> GSHTAEEDMEDDTSWRSEATFQFTVERFSRLSESVLSPPCFVRNLPWKIMVMPRFYPDRPHQKSVGFFLQCNAESDSTSWSCHAQAVLKIINYRDDEKSFSRRISHLFFHKENDWGFSNFMAWS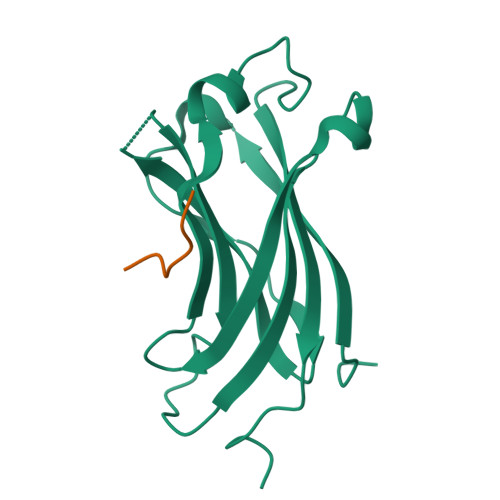EVTDPEKGFIDDDKVTFEVFVQADAPHGVAW;> YSQPSTSSSI> MGSSHHHHHHSSGRENLYFQGHMNGDQNSDAYAQEKQDFVQHFSQIVRVLTEDEMGHPEIGDAIARLKEVLEYNTIGGKYNRGLTVVVAFRELVEPRKQDADSLQRAWTVGWCVELLQAFFLVADDIMDSSLTRRGQICWYQKPGVGLDAINDANLLEACIYRLLKLYCREQPYYLNLIELFLQSSYQTEIGQTLDLLTAPQGNVDLVRFT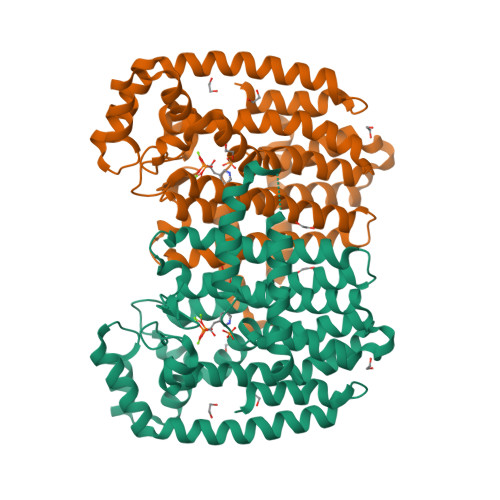EKRYKSIVKYKTAFYSFYLPIAAAMYMAGIDGEKEHANAKKILLEMGEFAQIQDDYLDLFGDPSVTGKIGTDIQDNKCSWLVVQCLQRATPEQYQILKENYGQKEAEKVARVKALYEELDLPAVFLQYEEDSYSHIMALIEQYAAPLPPAVFLGLARKIYKRRK> MKKIIYIATIGITLLTTSCDDFLDRQVPQGIVTGDQIASPEYVDNLVISAYAIWATGDDINSSFSLWNYDVRSDDCYKGGSGTEDGGVFNALEISKGINTTDWNINDIWKRLYQCITRANTALQSLDQMDEKTYPLKNQRIAEM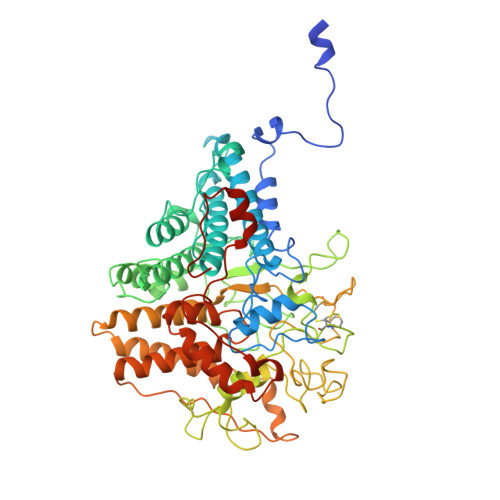RFLRGHAHFMLKQLFKKIVIVNDENMEPDAYNELSNTTYTNDEQWQKIADDFQFAYDNLPEVQIEKGRPAQAAAAAYLAKTYLYKAYRQDGADNALTGINEEDLKQVVKYTDPLIMAKGGYGLETDYSMNFLPQYENGAESVWAIQYSINDGTYNGNLNWGMGLTTPQILGCCDFHKPSQNLVNAFKTDSQGKPLFSTYDNENYEVATDNVDPRLFHTVGMPGFPYKYNEGYIIQKNDDWSRSKGLYGYYVSLKENVDPDCDCLKKGSYWASSLNHIVIRYADVLLMRAEALIQLNDGRITDAISLINEVRSRAAGSTMLIFNYKEDYGVNFKVTPYDLKAYAQDEAMKMLKWERRVEFGMESSRFFDLVRWGEAKDVINAYYVTEASRCSIYKNAGFTENKNEYLPVPFEQISASNGNYTQNFGWAAAAHHHHHH>MFRPGLEGVPATLSSISFVDGQRGVLEYRGISIEQLAQQSSFLETAYLLIWGHLPTQQELTEFEHEIRYHRRIKFRIRDMMKCFPDSGHPMDALQASAAALGLFYSRRALDDPEYIRAAVVRLLAKIPTMVAAFQLIRKGNDPIQPRDELDYAANFLYMLTEREPDPVAARIFDICLTLHAEHTINASTFSAMVTASTLTDPYAVVASAVGTLAGPLHGGANEEVLDMLEAIGSVENVEPYLDHCIATKTRIMGFGHRVYKVKDPRAVILQNLAEQLFDIFGHDPYYEIAVAVEKAAAERLSHKGIYPNVDFYSGLVYRKLGIPSDLFTPVFAIARVAGWLAHWKEQLNENRIFRPTQIYTGSHNLDYTPIADRDLAIESDLEHHHHHH[6x]

Here we report the discovery of a natural protein, citrate synthase from the cyanobacterium Synechococcus elongatus, which self-assembles into Sierpiński triangles. Bacterial citrate synthase (CS) proteins are homo-oligomeric enzymes that can assemble into dimers and hexamers. CS catalyses the condensation of acetyl-CoA and oxaloacetate to citrate as the first step in the tricarboxylic acid cycle. Using cryo-electron microscopy, we reveal how the fractal assembles from a hexameric building block.

An interaction between the residue E6 from one monomer and H369 of the other establishes an important contact, and mutating either E6 or H369 to alanine or deleting amino acids 2–6 (Δ2–6 SeCS) abolishes the formation of fractals. To understand how this interface forms, we compared the geometry of a variant that could only assemble into hexamers (Δ2–6 SeCS) to that of a hexamer within the 18mer. We extracted a hexamer from the 18mer structure, aligned its free corner dimer onto one dimer of Δ2–6 SeCS and then compared the positions of the two unaligned dimers between the structures. This analysis revealed that the two dimers engaging in fractal connections undergo a small clockwise rotation relative to their conformation within a free hexamer, which subtly breaks the D3 symmetry of the hexameric building block within the fractal. Comparing this structure to the one of a free hexamer (Δ2–6 SeCS) revealed that the CS dimers within the hexamer undergo an anticlockwise rotation after binding to citrate. This rigid-body rotation is well known from other CS enzymes. It takes place following substrate binding and pushes CS from an open conformation (which corresponds to the conformation in the Δ2–6 SeCS structure) into a closed form in which catalysis takes place.>[6x]MTSAEMTSPNNNSEHQAIAKMRTMIEGFDDISHGGLPIGRSTLVSGTSGTGKTLFSIQFLYNGIIEFDEPGVFVTFEETPQDIIKNARSFGWDLAKLVDEGKLFILDASPDPEGQEVVGGFDLSALIERINYAIQKYRARRVSIDSVTSVFQQYDASSVVRRELFRLVARLKQIGATTVMTTERIEEYGPIARYGVEEFVSDNVVILRNVLEGERRRRTLEILKLRGTSHMKGEYPFTITDHGINIFPLGAMRLTQRSSNVRVSSGVVRLDEMCGGGFFKDSIILATGATGTGKTLLVSRFVENACANKERAILFAYE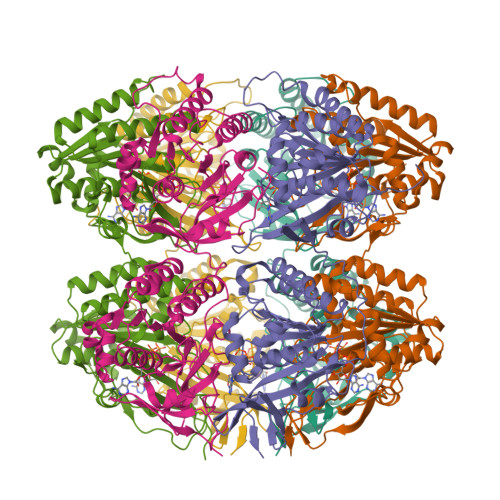ESRAQLLRNAYSWGMDFEEMERQNLLKIVCAYPESAGLEDHLQIIKSEINDFKPARIAIDSLSALARGVSNNAFRQFVIGVTGYAKQEEITGLFTNTSDQFMGAHSITDSHISTITDTIILLQYVEIRGEMSRAINVFKMRGSWHDKAIREFMISDKGPDIKDSFRNFERIISGSPTRITVDEKSELSRIVRGVQEKGPESHHHHHH> HKCDITLQEI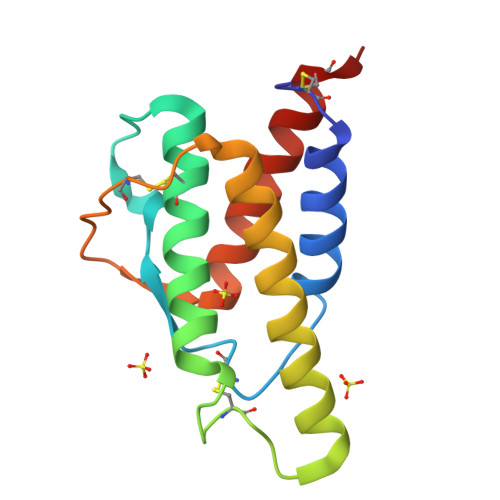IKTLNSLTEQKTLCTELTVTDIFAASKNTTEKETFCRAATVLRQFYSHHEKDTRCLGATAQQFHRHKQLIRDLKALDRNLWGLAGLNSCPVKEANQSTLENFLERLKTIMREKYSKCSS>[4x]MGSSHHHHHHSSGRENLYFQGMELLKHLSQRQYIDGEWVESANKNTRDIINPYN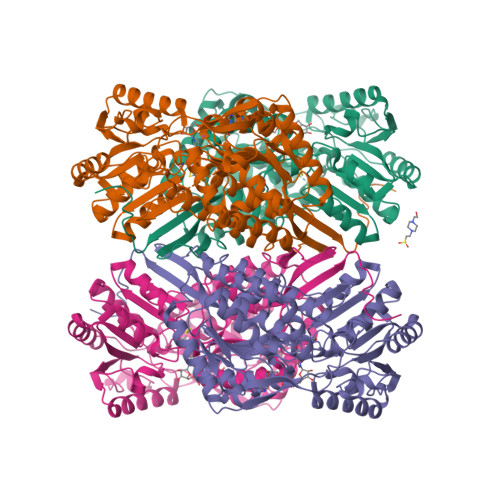QEVIFTVSEGTKEDAERAILAARRAFESGEWSQETAETRGKKVRAIADKIKEHREALARLETLDTGKTLEESYADMDDIHNVFMYFAGLADKDGGEMIDSPIPDTESKIVKEPVGVVTQITPWNYPLLQASWKIAPALATGCSLVMKPSEITPLTTIRVFELMEEVGFPKGTINLILGAGSEVGDVMSGHKEVDLVSFTGGIETGKHIMKNAANNVTNIALELGGKNPNIIFDDADFELAVDQALNGGYFHAGQVCSAGSRILVQNSIKDKFEQALIDRVKKIKLGNGFDADTEMGPVISTEHRNKIESYMDVAKAEGATIAVGGKRPDRDDLKDGLFFEPTVITNCDTSMRIVQEEVFGPVVTVEGFETEQEAIQLANDSIYGLAGAVFSKDIGKAQRVANKLKLGTVWINDFHPLFAQAPWGGYKQSGIGRELGKEGLEEYLVSKHILTNTNPQLVNWFSK> MLAVPAAR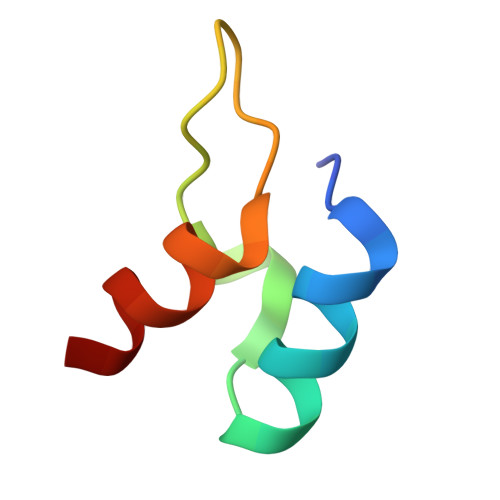KLARELGIPIEEVPGSGPLGRVRVEDVRAYAER> PQII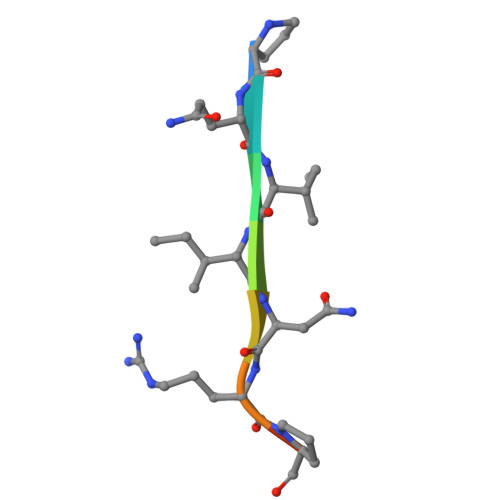NRPQN>SHMAHQDALPRLPVPPLQQSLDYYLKALQPIVSEEEWAHTKQLVDEFQTSGGVGERLQKGLERRAKKMENWLSEWWLKTAYLQFRQPVVIYSSPGVILPKQDFVDLQGQLRFAAKLIEGVLDFKSMIDNETLPVEFLGGQPLCMNQYYQILSSCRVPGPKQDSVVNFLKSKRPPTHITVVHNYQFFELDVYHSDGTPLTSDQIFVQLEKIWNSSLQSNKEPVGILTSNHRNTWAKAYNNLIKDKVNRESVNSIQKSIFTVCLDKQVPRVSDDVYRNHVAGQMLHGGGSKFNSGNRWFDKTLQFIVAEDGSCGMVYEHAAAEGPPIVALVDHVMEYTKKPELVRSPMVPLPMPKKLRFNITPEIKNDIEKAKQNLSIMIQDLDIMMLTFHHFGKDFPKSEKLSPDAFIQVALQLAYYRIYGQACATYESASLRMFHLGRTDTIRSASIDSLAFVKGMGDSTVPEQQKVELLRKAVQAHRAYTDRAIRGEAFDRHLLGLKLQAIEDLVSMPDIFMDTSYAIAMHFNLSTSQVPAKTDCVMFFGPVVPDGYGICYNPMEAHINFSVSAYNSCAETNAARMAHYLEKA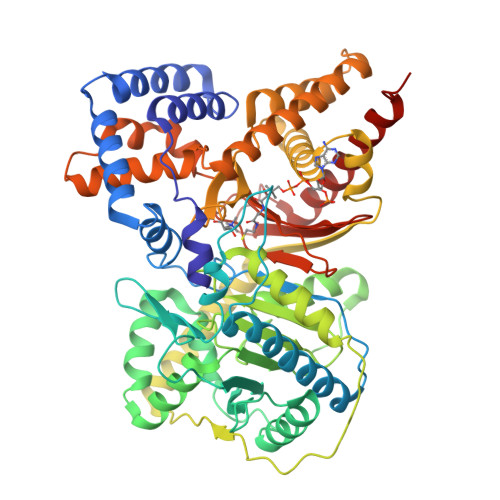LLDMRTLLQNHPRAK[2x]>[2x]ASPAANAIAYIVDGMGQTQISAARYLNAYKTAPERFPLNVSPAETPTGFDAFSSRGSMTTFPDDPYETTTDSAAAATAFASGVKTYNGAIGGVQTSGGGFQRVDTVLERASAQGYATGLITTTEATHATPAAFAAHVEDRGNQTEIARQYIEETQPDVILGGQRRDFEADASNGGTLVDAARDNGYTIAETAAELDAVDDPPVLGLFSQESHLD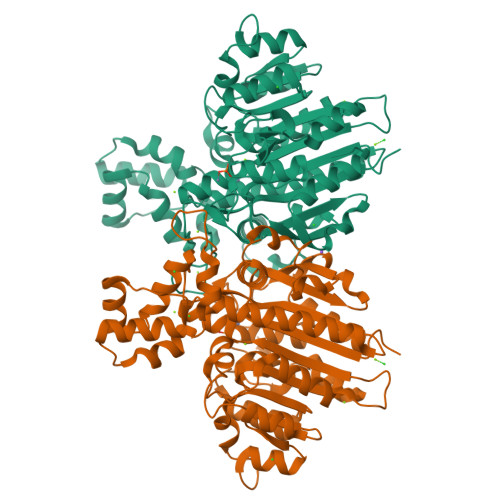YYLDRKNDPENTQPNLDAMVDAGVDLLSSAGDPDKGFFLLVESGRVDHAGHANYPAQVAEQYEATQVAGQLVEYAETTAEPTFLVSTGDHECGGLTLGRDSPYEVEYDVLAAQKATTSRLRDLLAGVRSADELESIVAAHTGITALTDREVAKLRDAPGSISTILAERAGIAFTTDGHTGTDVPVFAHGPNAARFDAARDNTAVADALAAALGVSLQ>QIMEPHDTLS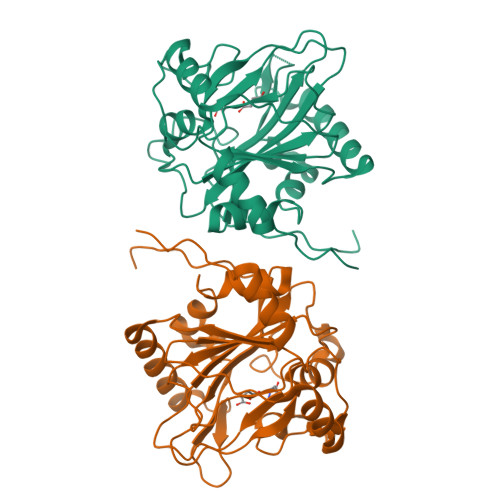PAQVDEYRKNGFLVQEHVFDEEEIELLRAEAAQEFASGGERVTVEQNTGIVRGVHGCHLYSEVFGRLVRSPRLLPIARQLLRDDVYVHQFKINAKRAFKGEVWEWHQDYTFWHHEDGMPAPRALSAAIFLDEVTEFNGPLTFVPGGHGSGMIDADVKGEGWANTLTASLKYSLDVETMRGLIERNGMVAPKGPRGSVLWFDANIPHSSVPNISPFDRGLVLITYNSVENKTDVTRGTRPEWLAARDFTPLTALQATSF[2x]>MAIAQLATEYVFSDFLLKEPTEPKFKGLRLELAVDKMVTCIAVGLPLLLISLAFAQEISIGTQISCFSPSSFSWRQAAFVDSYCWAAVQQKNSLQSESGNLPLWLHKFFPYILLLFAILLYLPPLFWRFAAAPHICSDLKFIMEELDKVYNRAIKAAKSARDLDMRDGACSVPGVTENLGQSLWEVSESHFKYPIVEQYLKTKKNSNNLIIKYISCRLLTLIIILLACIYLGYYFSLSSLSDEFVCSIKSGILRNDSTVPDQFQCKLIAVGIFQLLSVINLVVYVLLAPVVVYTLFVPFRQKTDVLKVYEILPTFDVLHFKSEGYNDLSLYNLFLEENISEVKSYKCLKVLENIKSSGQGIDPMLLLTNLGMIKMD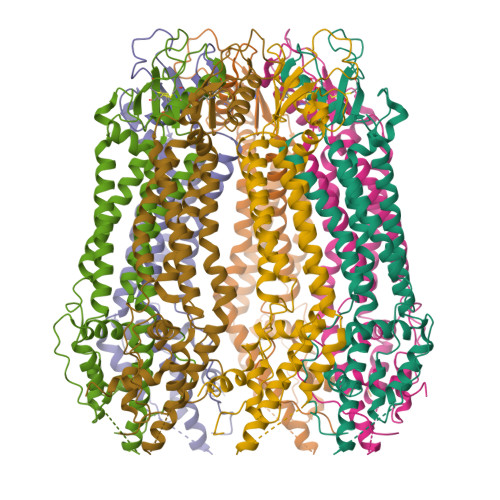VVDGKTPMSAEMREEQGNQTAELQGMNIDSETKANNGEKNARQRLLDSSCLEWSHPQFEK[7x]> MAQETYFYGQGEIDAAPIVNGVLGKWRWIQDVSAMSIQLAVEKVEHKESYSGQKALVRSFPIGKTATVNITLHSIGPDNLALTLYGKVVAKAAGSVTGEVLPADLVAGDVI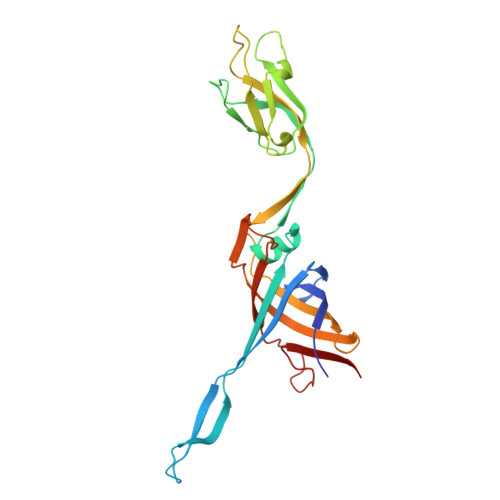RLANFGVSELVITDSASSPAPLDPQYYALRADGAYGEVQLLGLPTPAPTQPFKAAYEYAATKQVGMFTAPQPTVALRYKGINLAEGGAPVIVELYKVATDPLQELALISDGNTVAGMQISGGILLDTSKPDTGDLGRFGRIIQLG>MRISICKMKKDYRKKYRKYVRSRFQCIEDRNARLGESVSLNKRYTRLRLIKEHRSQQEREQELLAIGKTKTCESPVSPIKMELLFDPDDEHSEPVHTVVFQGAAGIGKTILARKMMLDWASGTLYQDRFDYLFYIHCREVSLVTQRSLGDLIMSCCPDPNPPIHKIVRKPSRILFLMDGFDELQGAFDEHIGPLCTDWQKAERGDILLSSLIRKKLLPEASLLITTRPVALEKLQHLLDHPRHVEILGFSEAKRKEYFFKYFSDEAQARAAFSLIQENEVLFTMCFIPLVCWIVCTGLKQQMESGKSLAQTSKTTTAVYVFFLSSLLQPRGGSQEHGLCAHLWGLCSLAADGIWNQKILFEESDLRNHGLQKADVSAFLRMNLFQKEVDCEKFYSFIHMTFQEFFAAMYYLLEEEKEGRTNVPGSRLKLPSRDVTVLLENYGKFEKGYLIFVVRFLFGLVNQERTSYLEKKLSCKISQQIRLELLKWIEVKAKAKKLQIQPSQLELFYCLYEMQEEDFVQRAMDYFPKIEINLSTRMDHM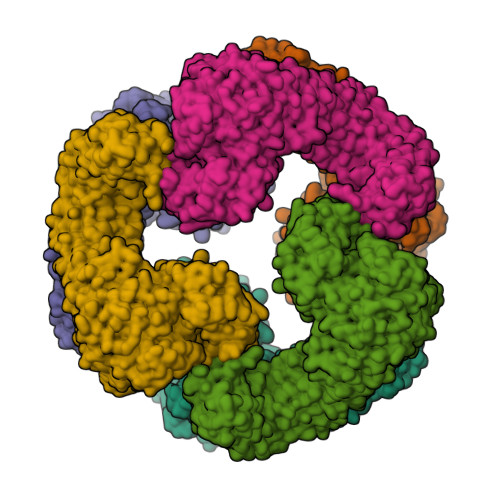VSSFCIENCHRVESLSLGFLHNMPKEEEEEEKEGRHLDMVQCVLPSSSHAACSHGLVNSHLTSSFCRGLFSVLSTSQSLTELDLSDNSLGDPGMRVLCETLQHPGCNIRRLWLGRCGLSHECCFDISLVLSSNQKLVELDLSDNALGDFGIRLLCVGLKHLLCNLKKLWLVSCCLTSACCQDLASVLSTSHSLTRLYVGENALGDSGVAILCEKAKNPQCNLQKLGLVNSGLTSVCCSALSSVLSTNQNLTHLYLRGNTLGDKGIKLLCEGLLHPDCKLQVLELDNCNLTSHCCWDLSTLLTSSQSLRKLSLGNNDLGDLGVMMFCEVLKQQSCLLQNLGLSEMYFNYETKSALETLQEEKPELTVVFEPSWGSGGDYKDDDDK[6x]>GSHMLRISQEALTFDDVLLIPGYSEVLPKDVSLKTRLTRGIELNIPLVSAAMDTVTEARLAIAMAQEGGIGIIHKNMGIEQQAAEVRKVKKHETAIVRDPVTVTPSTKIIELLQMAREYGFSGFPVVEQGELVGIVTGRDLRVKPNAGDTVAAIMTPKDKLVTAREGTPLEEMKAKLYENRIEKMLVVDENFYLRGLVTFRDIEKAKTYPLASKDEQGRLRVGAAVGTGADTGERVAALVAAGVDVVVVDTAHGHSKGVIERVRWVKQTFPDVQVIGGNIATAEAAKALAEAGADAVKVGIGPGSICTTRIVAGVGVPQISAIANVAAALEGTGVPLIADGGIRFSGDLAKAMVAGAYCVMMGSMFAGTEEAPGEIELFQGRSYKSYRGMGSLGAMSGSQGSSDRYFQDASAGAEKLVPEGIEGRVPYKGALSAIVHQLMGGLRAAMGY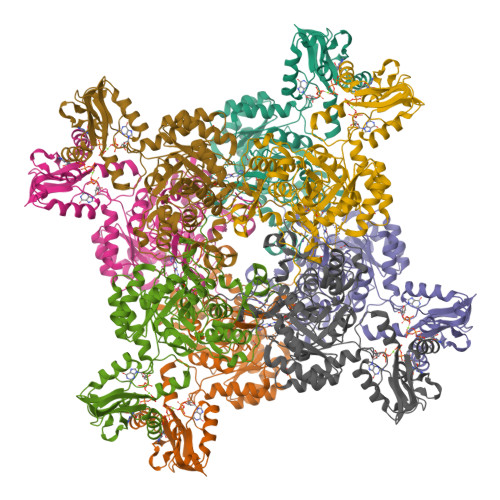TGSADIQQMRTQPQFVRITGAGMAESHVHDVQITKEAPNYRVG[2x]Pannexins are single-membrane large-pore channels that release ions and ATP upon activation. Three isoforms of pannexins 1, 2, and 3, perform diverse cellular roles and differ in their pore lining residues. Pannexin protomers retain structural and topological similarity to innexins, connexins, and volume-regulated anion channels but remain as single-membrane channels and participate in ion-conductance and ATP release. The PANX isoforms, PANX1, PANX2, and PANX3 harbor substitutions in the residues that control channel gating and can have architectural differences that form the basis for altered properties among the three isoforms.

We elucidated the structure of PANX1R217H (TM3) substitution to characterize the effects of this germline mutant and to understand the basis of its defective channel properties. The arginine residue at the 217 position (TM3) is highly conserved among vertebrate PANX1 orthologues and is buried amongst TM helices and does not display solvent access unlike the substitutions studied earlier. The structure was determined by cryo-EM to a resolution of 3.9 Å. Despite the lower resolution of the structure, it resembles PANX1WT globally, with subtle changes in extracellular domain (ECD), extracellular helix 1 (EH1), and the intracellular domain (ICD). Mutating arginine to histidine disrupts the H-bond interaction network within TMs 1 and 3. The G44 in TM1 that likely acts as a hinge point facilitates the TM1 bending and displacement as a consequence of R217H substitution. The displacement observed in TM1 translates to an outward movement of ECD that could facilitate greater flexibility of the pore lining residue W74 to constrict the channel. In comparison to the PANX1WT, the modeled side chain W74 has a χ2 torsion angle shift of nearly 80° towards the pore leading to a constriction of the pore diameter in the mutant PANX1. A comparison of normalized conductance to voltage for PANX1R217H and PANX1WT reveals altered voltage sensitivity (V50) of the mutant channel from around 40 mV for the PANX1WT to over 100 mV indicating reduced voltage sensitivity as a consequence of R217H mutation. Binding studies using MST display a significant decrease in ATP-γS binding in the PANX1R217H mutant compared to PANX1WT suggesting that mutant behaves differently than the PANX1WT and have reduced ability to bind to ATP-γS.

>MAIAQLATEYVFSDFLLKEPTEPKFKGLRLELAVDKMVTCIAVGLPLLLISLAFAQEISIGTQISCFSPSSFSWRQAAFVDSYCWAAVQQKNSLQSESGNLPLWLHKFFPYILLLFAILLYLPPLFWRFAAAPHICSDLKFIMEELDKVYNRAIKAAKSARDLDMRDGACSVPGVTENLGQSLWEVSESHFKYPIVEQYLKTKKNSNNLIIKYISCHLLTLIIILLACIYLGYYFSLSSLSDEFVCSIKSGILRNDSTVPDQFQCKLIAVGIFQLLSVINLVVYVLLAPVVVYTLFVPFRQKTDVLKVYEILPTFDVLHFKSEGYNDLSLYNLFLEENISEVKSYKCLKVLENIKSSGQGIDPMLLLTNLGMIKMDVVDGKTPMSAEMREEQGNQTAELQGMNIDSETKANNGEKNARQRLLDSSC[7x]(7S,10S,13S,17P)-10-(4-aminobutyl)-7-(3-aminopropyl)-17-(6-aminopyridin-3-yl)-20-chloro-13-[(1H-indol-3-yl)methyl]-12-methyl-6,7,9,10,12,13,15,16-octahydropyrido[2,3-b][1,5,8,11,14]benzothiatetraazacycloheptadecine-8,11,14(5H)-trione 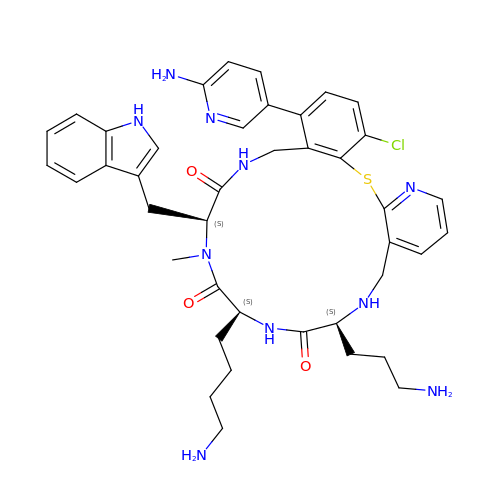| C41 H49 Cl N10 O3 S | BDHOZQIIBFIAMB-IMKBVMFZSA-N>[6x]MVIGVPKEIKTLENRVALTPGGVESLVRRGHTVLVERGAGEGSGLSDAEYARAGAELVGREEAWGAEMVVKVKEPLPEEYGFLREGLILFTYLHLAADRGLTEAMLRSGVTGIAYETVQLPDGTLPLLVPMSEVAGRMAPQVGAQFLEKPKGGRGVLLGGVPGVAPASVVILGGGTVGTNAAKIALGMGAQVTILDVNHKRLQYLDDVFGGRVITLTATEANIKKSVQHADLLIGA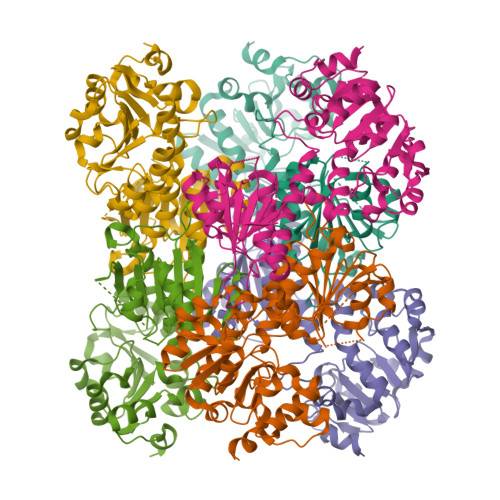VLVPGAKAPKLVTRDMLSLMKEGAVIVDVAVDQGGCVETIRPTTHAEPTYVVDGVVHYGVANMPGAVPRTSTFALTNQTLPYVLKLAEKGLDALLEDAALLKGLNTHKGRLTHPGVAEAFGLPYTPPEEALRG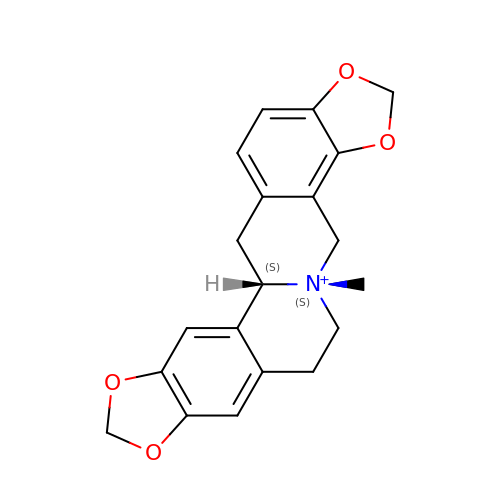(5S,12bS)-5-methyl-6,7,12b,13-tetrahydro-2H,4H,10H-[1,3]dioxolo[4,5-g][1,3]dioxolo[7,8]isoquinolino[3,2-a]isoquinolin-5-ium | C20 H20 N O4 | GBUUKFRQPCPYPW-KKSFZXQISA-N>MALKA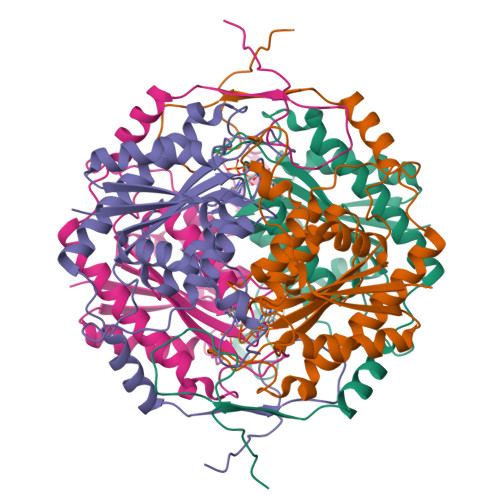LILNTTLRRSPSRSQTQGLIDKAVPLYEKEGIETEVVRVIDHDIEQEYWDDYDDWNAGEKARREDEWPWLLEKIREADILVIATPITLNMCTSAAHVILEKLNLMDELNGDTKQFPLYNKVAGLLMCGNEDGAHHVAGTVLNNLGRLGYSVPPNAAAYWLGPAGTGPGYIEGKGDRHFHTNKLIRFMVANTSHLARMLQETPYTTDLEACAQAAREESDDVFAIRVNVNTPAIRYKRFQKLGEVKVEESQLG[8x]> ATSDSNMLLNYVPVYVMLPLGVVNVDNVFEDPDGLKEQLLQLRAAGVDGVMVDV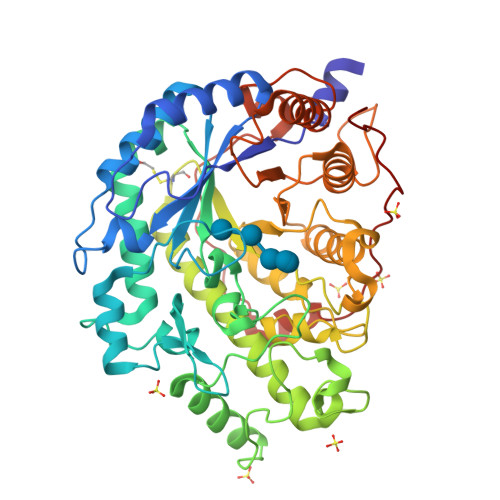WWGIIELKGPKQYDWRAYRSLLQLVQECGLTLQAIMSFHQCGGNVGDIVNIPIPQWVLDIGESNHDIFYTNRSGTRNKEYLTVGVDNEPIFHGRTAIEIYSDYMKSFRENMSDFLESGLIIDIEVGLGPAGELRYPSYPQSQGWEFPGIGEFQCYDKYLKADFKAAVARAGHPEWELPDDAGKYNDVPESTGFFKSNGTYVTEKGKFFLTWYSNKLLNHGDQILDEANKAFLGCKVKLAIKVSGIHWWYKVENHAAELTAGYYNLNDRDGYRPIARMLSRHHAILNFSCLEMRDSEQPSDAKSGPQELVQQVLSGGWREDIRVAGENALPRYDATAYNQIILNARPQGVNNNGPPKLSMFGVTYLRLSDDLLQKSNFNIFKKFVLKMHADQDYCANPQKYNHAITPLKPSAPKIPIEVLLEATKPTLPFPWLPETDMKVDG> SNIDGMKLFLQHCKTCHGVDGNPTDLGEGLGARKFADAEWQAKTSDERIIEQINEGTPEMMMPFKEK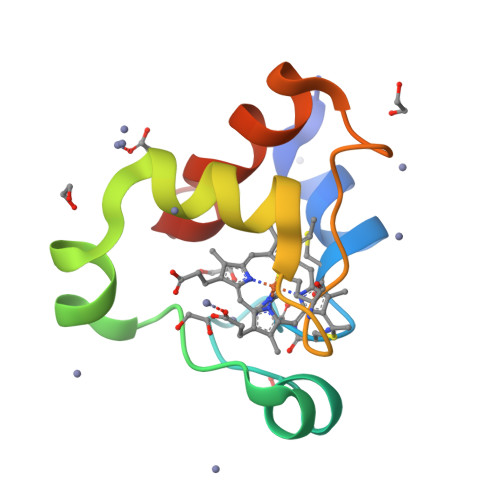LTPEEVKALVPVVRGFKK> ADKELKFLVVGNGGTGKSTVRNLLKELGFNN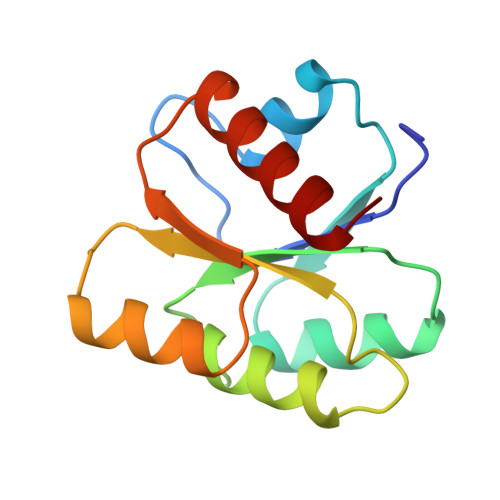VEDAEDGVDALNKLQAGGYGFVISDWNMPNMDGLELLKTIRADGAMSALPVLMVTAEAKKENIIAAAQAGASGYVVKPFTAATLEEKLNKIFEKLGM>[5x]GCGGAUUUAGCUCAGUUGGGA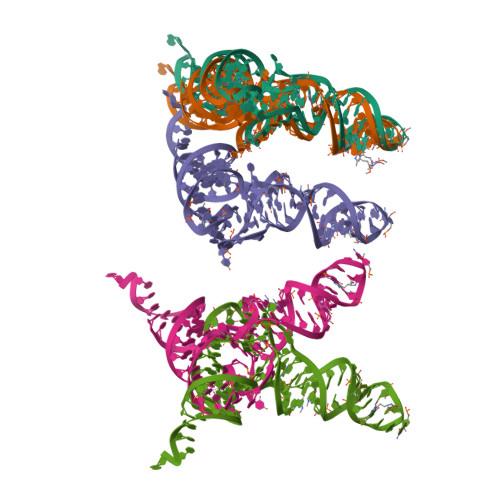GAGCGCCAGACUGAAGAUCUGGAGGUCCUGUGUUCGAUCCACAGAAUUCGCACCA> MQFLNMFFFDIYPYIAGAVFLIGSWLRYDYGQYTWRAASSQMLDRKGMNLASNLFHIGILGIFVGHFFGMLTPHWMAAAWLPIEVKQKMAMFAGGASGVLCLIGGVLLLKRRLFSPRVRATTTGADILILSLLVIQCALGLLTIPFSAQHMDGSEMMKLVGWAQSVVTFHGGASQHLDGVAFIFRLHLVLGMTLFLLFPFSRLIHIWSVPV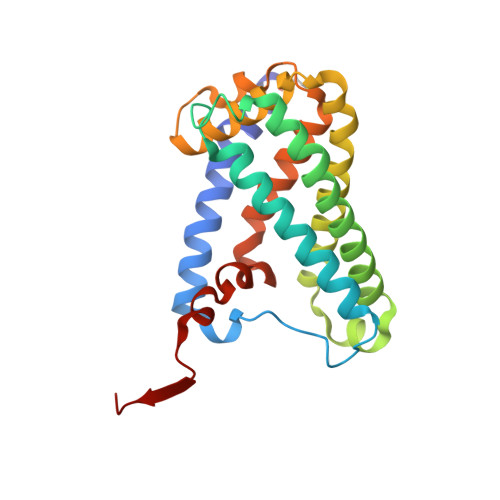EYLTRKYQLVRARH L-Serine, N-[[3-hydroxy-2-methyl-5-[(phosphonooxy)methyl]-4-pyridinyl]methylene] | C11 H14 N2 O8 P 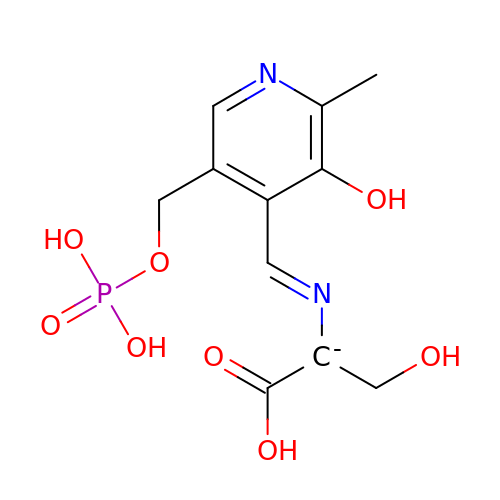| JFLJYKRWFQAEDK-QLKAYGNNSA-N> MAFNFGAPSGTSGTAAATAAPAGGFGGFGTTSTTAGSAFSFSAPTNTGTTGLFGGTQNKGFGFGTGFGTTTGTSTGLGTGLGTGLGFGGFNTQQQQQTTLGGLFSQPTQAPTQSNQLINTASALSAPTLLGDERDAILAKWNQLQAFWGTGKGYFNNNIPPVEFTQENPFCRFKAVGYSCMPSNKDEDGLVVLVFNKKETEIRSQQQQLVESLHKVLGGNQTLTVNVEGTKTLPDDQTEVVIYVVERSPNGTSRRVPATTLYAHFEQANIKTQLQQLGVTLSMTRTELSPAQIKQLLQNPPAGVDPIIWEQAKVDNPDSEKLIPVPMVGFKELLRRLKVQDQMTKQHQTRLDIISEDISELQKNQTTSVAKIAQYKRKLMDLSHRTLQVLIKQEIQRKSGYAIQADEEQLRVQLDTIQGELNAPTQFKGRLNELMSQIRMQNHFGAVRSEERYYIDADLLR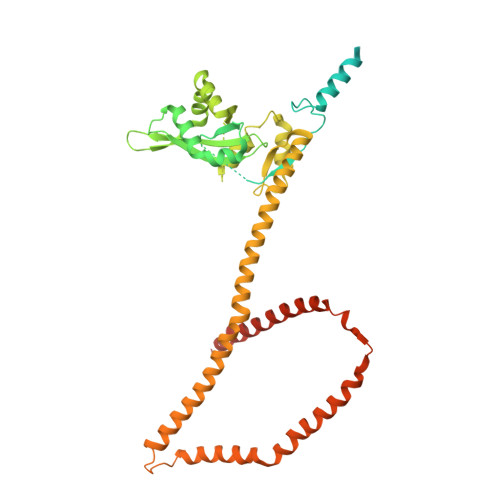EIKQHLKQQQEGLSHLISIIKDDLEDIKLVEHGLNETIHIRGGVFS> AKLVRLPGLIDVHVHLREPGGTHKEDFASGTAAALAGGITMVCAMPNTRPPIIDAPALALAQKLAEAGARCDFALFLGASSENAGTLGTVAGSAAGLKLYLANATTNSSHGVTSVVQWMEHFETWPSHLPIVAHAEEQTVAAV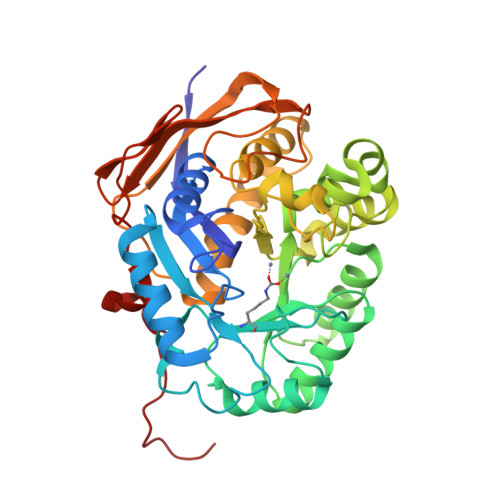LMVAQLTQRSVHICHVARKEEILLIKAAKARGLPVTCEVAPHHLFLSHDDLERLGPGKGEVRPELGSRQDVEALWENMAVIDCFASDHAPHTLEEKCGSRPPPGFPGLETMLPLLLTAVSEGRLSLDDLLQRLHHNPRRIFHLPPQEDTYVEVDLEHEWTIPSHMPFSKAHWTPFEGQKVKGTVRRVVLRGEVAYIDGQVLVPPGYGQDVRKWPQGAVPQLPPSAPAA PAROMOMYCIN (RING 2) | C6 H14 N2 O2 | 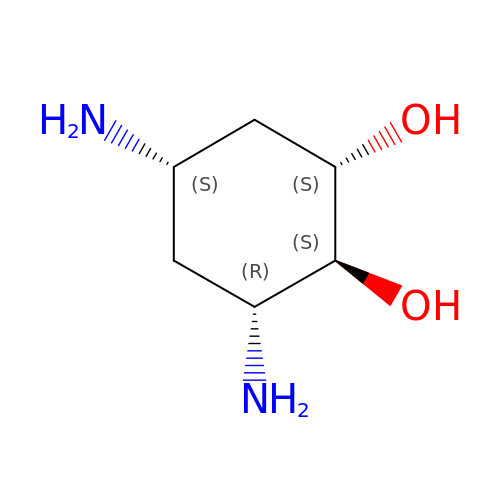QOLDZWBHLDQIJR-FSIIMWSLSA-N>[2x]MAHHHHHHMPSLFDPLTIGDLTLANRIIMAPLTRARAGDTRTPNALMARYYAERASAGLIISEATSVTPQGVGYASTPGIWSPEQVDGWRLVTDAVHAAGGRIFLQLWHVGRVSDPVFLDGALPVAPSAIAPGGHVS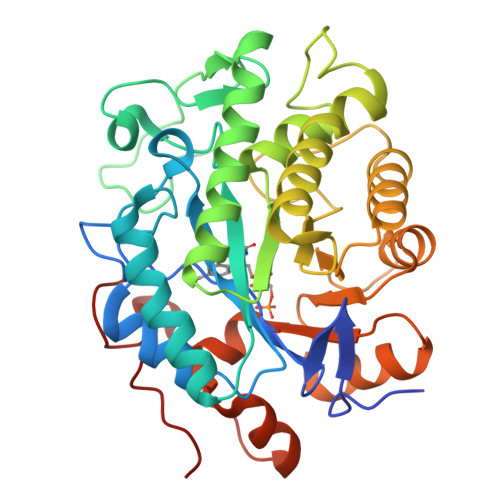LVRPQRPYVTPRALELDEIPGVVAAFRRGAENARAAGFDGVEVHGANGYLLDQFLQDSANRRTDAYGGSIENRARLLLEVVDAAIDVWSAARVGVHLAPRGDAHTMGDSDPAATFGHVARELGRRRIAFLFARESFGGDAIGQQLKAAFGGPFIVNENFTLDSAQAALDAGQADAVAWGKLFIANPDLPRRFKLNAPLNEPNAATFYAQGEVGYTDYPALESAA>MSLRDTQTQLRNEMIYSVFVRNYSEAGNFAGVTADLQRIKDLGTDILWLLPINPIGEVNRKGTLGSPYAIKDYRGINPEYGTLADFKALTDRAHELGMKVMLDIVYNHTSPDSVLATEHPEWFYHDADGQLTNKVGDWSDVKDLDYGHHELWQYQIDTLLYWSQFVDGYRCDVAPLVPLDFWLEARKQVNAKYPETLWLAESAGSGFIEELRSQGYTGLSDSELYQAFDMTYDYDVFGDFKDYWQGRSTVERYVDLLQRQDATFPGNYVKMRFLENHDNARMMSLMHSKAEAVNNLTWIFMQRGIPLIYNGQEFLAEHQPSLFDRDTMVADRHGDVTPLIQKLVTIKQLPLLRAADYQLAVVEEGIVKITYRAAGEALTAWIPLKGQVTAVATKLAAGSYQNLLTDGPTEVVDGKLTVDGQPVLIKYVTNTAVTKVADQSNEGHHHHHH[4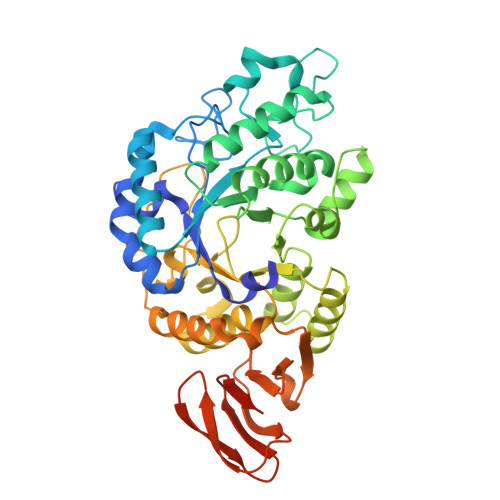x]> MFINPRNVSNTFLQEPLRHSS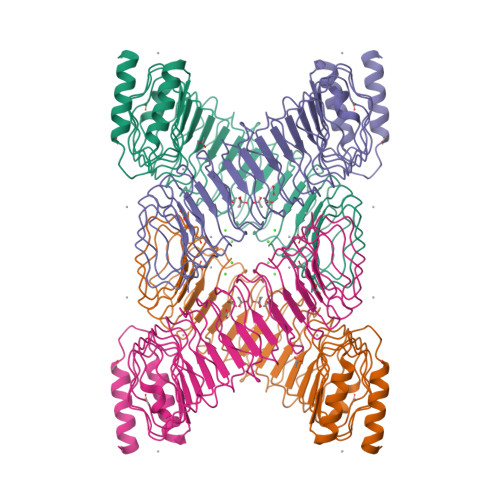NLTEMPVEAENVKSKTEYYNAWSEWERNAPPGNGEQREMAVSRLRDCLDRQAHELELNNLGLSSLPELPPHLESLVASCNSLTELPELPQSLKSLLVDNNNLKALSDLPPLLEYLGVSNNQLEKLPELQNSSFLKIIDVDNNSLKKLPDLPPSLEFIAAGNNQLEELPELQNLPFLTAIYADNNSLKKLPDLPLSLESIVAGNNILEELPELQNLPFLTTIYADNNLLKTLPDLPPSLEALNVRDNYLTDLPELPQSLTFLDVSENIFSGLSELPPNLYYLNASSNEIRSLCDLPPSLEELNVSNNKLIELPALPPRLERLIASFNHLAEVPELPQNLKQLHVEYNPLREFPDIPESVEDLRMNSHLAEVPELPQNLKQLHVETNPLREFPDIPESVEDLRMNSERVVDPYEFAHETTDKLEDDVFEHHHHHH>[4x]MSSSGTPDLPVLLTDLKIQYTKIFINNEWHDSVSGKKFPVFNPATEEELCQVEEGDKEDVDKAVKAARQAFQIGSPWRTMDASERGRLLYKLADLIERDRLLLATMESMNGGKLYSNAYLNDLAGCIKTLRYCAGWADKIQGRTIPIDGNFFTYTRHEPIGVCGQIIPWNFPLVMLIWKIGPALSCGNTVVVKPAEQTPLTALHVASLIKEAGFP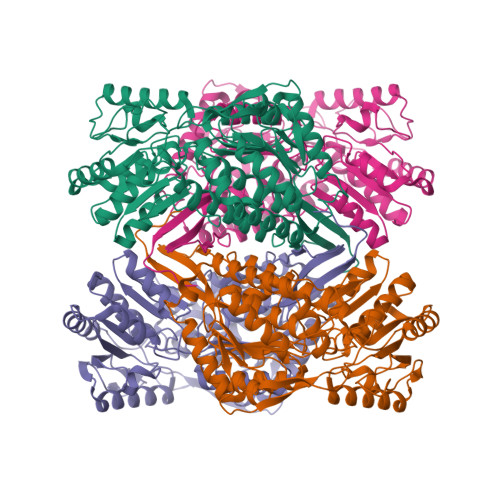PGVVNIVPGYGPTAGAAISSHMDIDKVAFTGSTEVGKLIKEAAGKSNLKRVTLELGGKSPCIVLADADLDNAVEFAHHGVFYHQGQCCIAASRIFVEESIYDEFVRRSVERAKKYILGNPLTPGVTQGPQIDKEQYDKILDLIESGKKEGAKLECGGGPWGNKGYFVQPTVFSNVTDEMRIAKEEIFGPVQQIMKFKSLDDVIKRANNTFYGLSAGVFTKDIDKAITISSALQAGTVWVNCYGVVSAQCPFGGFKMSGNGRELGEYGFHEYTEVKTVTVKISQKNS N-(2-FLUOROPHENYL)-4-[(4-FLUOROPHENYL)SULFONYL]-2,3,4,5-TETRAHYDRO-1,4-BENZOXAZEPIN-6-AMINE | C21 H18 F2 N2 O3 S | 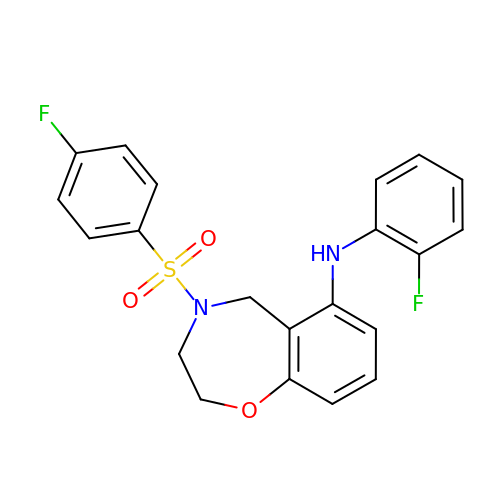HCJWPYDAKXNGHM-UHFFFAOYSA-N>MQKGRVKWFNAEKGYGFIEREGDTDVFVHYTAIN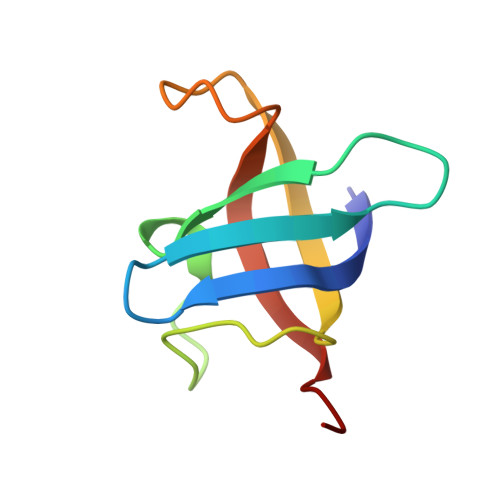AKGFRTLNEGDIVTFDVEPGRNGKGPQAVNVTVVEPARR[2x]>MDDLLQRVRRCEALQQPEWGDPSRLRDVQAYLRGSPALIRAGDILALRATLARVARGEALVVQCGDCAEDMDDHHAENVARKAAVLELLAGALRLAGRRPVIRVGRIAGQYAKPRSKPHEQVGEQTLPVYRGDMVNGREAHAEQRRADPQRILKGYAAARNIMRHLGWDAASGQEANASPVWTSHEMLLLDYELSMLREDEQRRVYLGSTHWPWIGERTRQVDGAHVALLAEVLNPVACKVGPEIGRDQLLALCERLDPRREPGRLTLIARMGAQKVGERLPPLVEAVRAAGHPVIWLSDPMHGNTIVAPCGNKTRLVRSIAEEVAAFRLAVS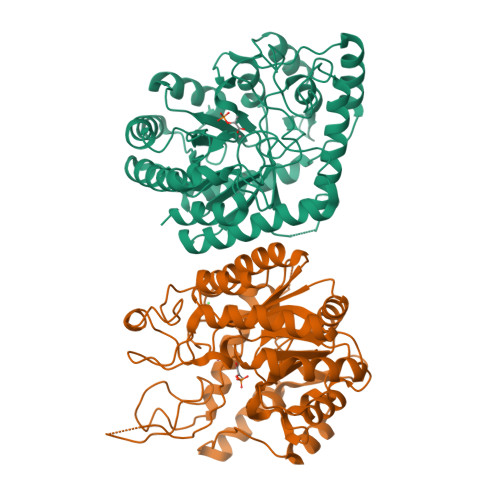GSGGVAAGLHLETTPDDVTECVADSSGLHQVSRHYTSLCDPRLNPWQALSAVMAWSGAEAIPSATFPLETVA[2x]> SDRPLSVHLNLGQKGNRKTSCPIKINQFEGHFMKLQADSNYLLSKEYEELKDVGRNQSCDIALLPENRGKNRYNNILPYDATRVKLSNVDDDPCSDYINASYIPGNNFRREYIVTQGPLPGTKDDFWKMVWEQNVHNIVMVTQCVEKGRVKCDHYWPADQDSLYYGDLILQMLSESVLPEWTIREFKICGEEQLDAHRLIRHFHYTVWPDHGVPETTQSL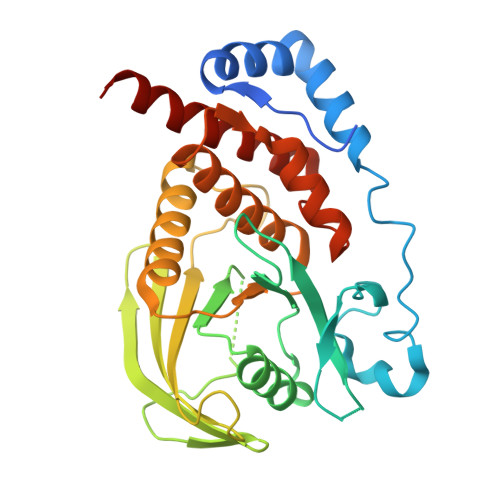IQFVRTVRDYINRSPGAGPTVVHCSAGVGRTGTFIALDRILQQLDSKDSVDIYGAVHDLRLHRVHMVQTECQYVYLHQCVRDVLRARKLRSEQ> GMYLKELSMMPGVSGDEGKVRDFIKSKIEGLVDNLYTDVLGNLIALKRGRDSSKKLLVSAHMDEVGFVVSKIEKDGKVSFLPVGGVDPRILPGKVVQVKNLKGVIGYRPIHLQRDEENTPPRFENLRIDFGFSSADEAKKYVSIGDYVSFVSDYIEKNGRAVGKAFDDRAGCSVLIDVLESGVSPAYDTYFVFTVQEETGLRGSAVVVEQLKPT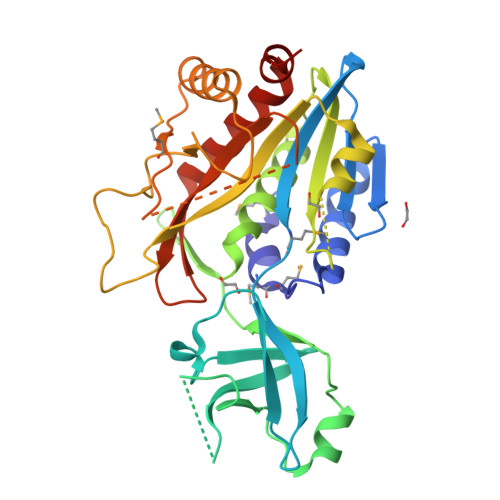CAIVVETTTAGDNPELEERKWATHLGDGPAITFYHRGYVIPKEIFQTIVDTAKNNDIPFQMKRRTAGGTDAGRYARTAYGVPAGVISTPARYIHSPNSIIDLNDYENTKKLIKVLVEEGKIVEVVS>MAIAHLATEYVFSDFLLKEPTEPKFKGLRLELAVDKMVTCIAVGLPLLLISLAFAQEISIGTQISCFSPSSFSWRQAAFVDSYCWAAVQQKSSLQSESGNLPLWLHKFFPYILLLFAILLYLPALFWRFSAAPHLCSDLKFIMEELDKVYNRAIKAAKSARDLDLRDGPGPPGVTENVGQSLWEISESHFKYPIVEQYLKTKKNSSHLIMKYISCRLVTFVVILLACIYLSYYFSLSSLSDEFLCSIKSGVLKNDSTIPDRFQCKLIAVGIFQLLSLINLIVYALLIPVVVYTFFIPFRQKTDILKVYEILPTFDVLHFKSEGYN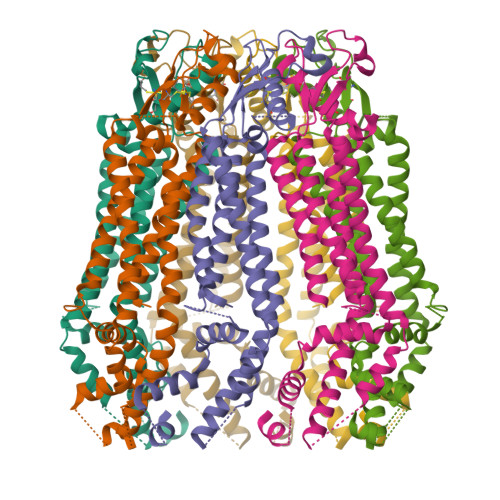DLSLYNLFLEENISELKSYKCLKVLENIKSNGQGIDPMLLLTNLGMIKMDIIDGKIPTSLQTKGEDQGSQRVEFKDLDLSSEAAANNGEKNSRQRLLNPSCGSAAAENLYFQGHHHHHH[7x]> GLNSSYVNGNTAGNLYNAGLFCESDGEVFFSNTNDNGRLYAMNIDGSNIHKLSNDTAMYINADKNYVYYVRNNNQKITSQTFFSYDRNSLCRIKR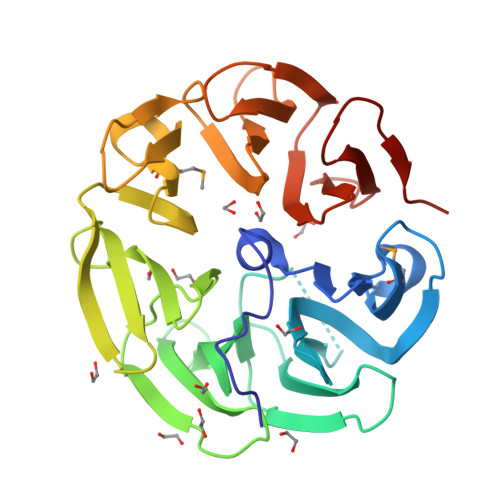NGHGSTVLDPDPCIYASLIGNYIYYLHYDTQTATSLYRIRIDGEEKKKIKNHYLFTCNTSDRYFYYNNPKNGQLYRYDTASQSEALFYDCNCYKPVVLDDTNVYYMDVNRDNAIVHVNINNPNPVVLTEANIEHYNVYGSLIFYQRGGDNPALCVVKNDGTGFKELAKGEFCNINVTSQYVYFTDFVSNKEYCTSTQNPDTIKALQP> GPTPEAPYASLTEIEHLVQSVCKSYRETCQLRLEDLLR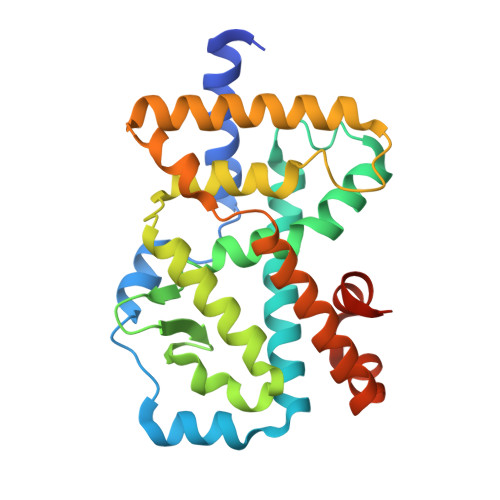QRSNIFSREEVTGYQRKSMWEMWERCAHHLTEAIQYVVEFAKRLSGFMELCQNDQIVLLKAGAMEVVLVRMCRAYNADNRTVFFEGKYGGMELFRALGCSELISSIFDFSHSLSALHFSEDEIALYTALVLINAHRPGLQEKRKVEQLQYNLELAFHHHLCKTHRQSILAKLPPKGKLRSLCSQHVERLQIFQHLHPIVVQAAFPPLYKELFSTTETESPVGLSK>MANLEIGKSILAAGVLTNYHDVGEGQPVILIHGSGPGVSAYANWRLTIPALSKFYRVIAPDMVGFGFTDRPENYNYSKDSWVDHIIGIMDALEIEKAHIVGNAFGGGLAIATALRYSERVDRMVLMGAAGTRFDVTEGLNAVWGYTPSIENMRNLLDIFAYDRSLV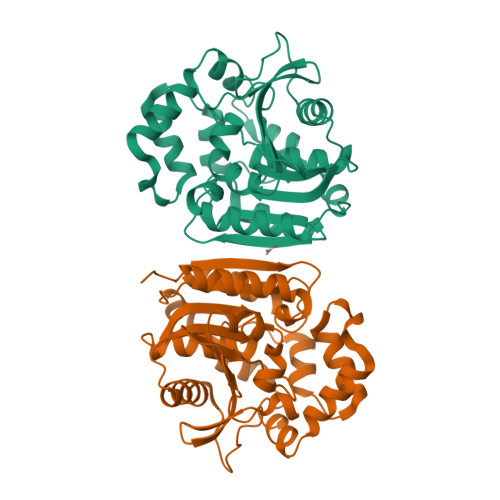TDELARLRYEASIQPGFQESFSSMFPEPRQRWIDALASSDEDIKTLPNETLIIHGREDQVVPLSSSLRLGELIDRAQLHVFGRCGHWTQIEQTDRFNRLVVEFFNEANTPKLVGRP[2x]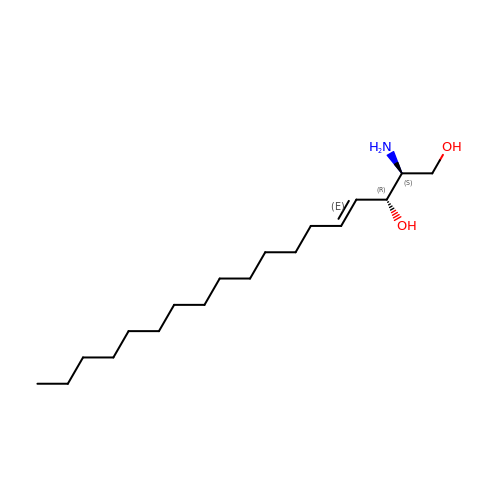(2S,3R,4E)-2-aminooctadec-4-ene-1,3-diol | C18 H37 N O2 | WWUZIQQURGPMPG-KRWOKUGFSA-N> MTGGMKPPARKPRILNSDGSSNITRLGLEKRGWLDDHYHDLLTVSWPVFITLITGLYLVTNALFALAYLASGDVIENARPGSFTDAFFF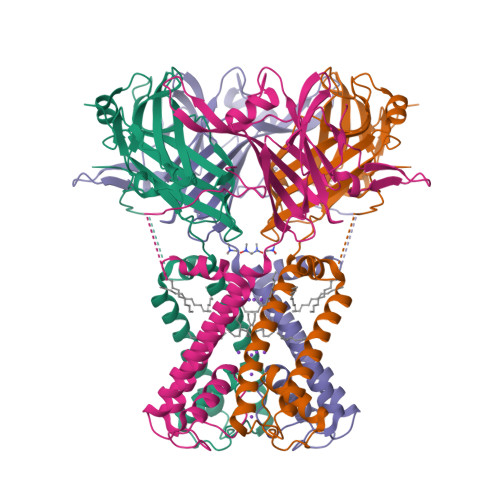SVQTMATIGYGKLIPIGPLANTLVTLEALCGMLGMAVAASLIYARFTRPTAGVLFSSRMVISDFEGKPTLMMRLANLRIEQIIEADVHLVLVRSEISQEGMVFRRFHDLTLTRSRSPIFSLSWTVMHPIDHHSPIYGETDETLRNSHSEFLVLFTGHHEAFAQNVHARHAYSSDEIIWGGHFVDVFTTLPDGRRALDLGKFHEIAQHHHHHH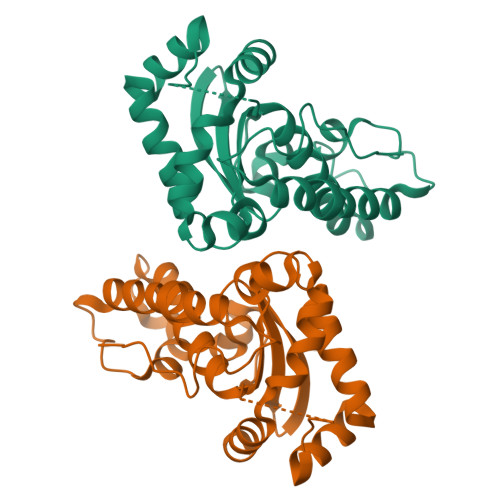>[2x]MAYTLPQLPYAYDALEPHIDARTMEIHHTKHHQTYVDNANKALEGTEFADLPVEQLIQQLDRVPADKKGALRNNAGGHANHSMFWQIMGQGQGQNGANQPSGELLDAINSAFGSFDAFKQKFEDAAKTRFGSGWAWLVVKDGKLDVVSTANQDNPLMGEAIAGVSGTPILGVDVWEHAYYLNYQNRRPDYLAAFWNVVNWDEVSKRYAAAK> MIRLYPEQLRAQLNEGLRAAYLLLGNDPLLLQESQDAVRQVAAAQGFEEHHTFSIDPNTDWNAIFSLCQAMSLFASRQTLLLLLPENGPNAAINEQLLTLTGLLHDDLLLIVRGNKLSKAQENAAWFTALANRSVQVTCQTPEQAQLPRWVAARAKQLNLELDDAANQVLCYCYEGNLLALAQALERLSLLWPDGKLTLPRVEQAVNDAAHFTPFHWVDALLMGKSKRALHILQQLRLEGSEPVILLRTLQRELLLLVNLKRQSAHTPLRALFDKHRVWQNRRGMMGEALNRLSQTQLRQAVQLLTRTELTLKQDYGQSVWAELEGLSLLLCHKPLADVFIDG;>GPHMSYQVLARKWRPQTFADVVGQEHVLTALANGLSLGRIHHAYLFSGTRGVGKTSIARLLAKGLNCETGITATPCGVCDNCREIEQGRFVDLIEIDAASRTKVEDTRDLLDNVQYAPARGRFKVYLIDEVHMLSRHSFNALLKTLEEPPEHVKFLLATTDPQKLPVTILSRCLQFHLKALDVEQIRHQLEHILNEEHIAHEPRALQLLARAAEGSLRDALSLTDQAIASGDGQVSTQAVSAMLGTLDDDQALSLVEAMVEANGERVMALINEAAARGIEWEALLVEMLGLLHRIAMVQLSPAALGNDMAAIELRMRELARTIPPTDIQLYYQTLLIGRKELPYAPDRRMGVEMTLLRALAFHPRMPLPEPEVPRQ[3x];> GPHMRWYPWLRPDFEKLVASYQAGRGHHALLIQALPGMGDDALIYALSRYLLCQQPQGHKSCGHCRGCQLMQAGTHPDYYTLAPEKGKNTLGVDAVREVTEKLNEHARLGGAKVVWVTDAALLTDAAANALLKTLEEPPAETWFFLATREPERLLATLRSRCRLHYLAPPPEQYAVTWLSREVTMSQDALLAALRLSAGSPGAALALFQGDNWQARETLCQALAYSVPSGDWYSLLAALNHEQAPARLHWLATLLMDALKRHHGAAQVTNVDVPGLVAELANHLSPSRLQAILGDVCHIREQLMSVTGINRELLITDLLLRIEHYLQPGVVLPVPHL;>[2x]GPHMKFTVEREHLLKPLQQVSGPLGGRPTLPILGNLLLQVADGTLSLTGTDLEMEMVARVALVQPHEPGATTVPARKFFDICRGLPEGAEIAVQLEGERMLVRSGRSRFSLSTLPAADFPNLDDWQSEVEFTLPQATMKRLIEATQFSMAHQDVRYYLNGMLFETEGEELRTVATDGHRLAVCSMPIGQSLPSHSVIVPRKGVIELMRMLDGGDNPLRVQIGSNNIRAHVGDFIFTSKLVDGRFPDYRRVLPKNPDKHLEAGCDLLKQAFARAAILSNEKFRGVRLYVSENQLKITANNPEQEEAEEILDVTYSGAEMEIGFNVSYVLDVLNALKCENVRMMLTDSVSSVQIEDAASQSAAYVVMPMRL

Clamp loaders are pentameric ATPases that place circular sliding clamps onto DNA, where they function in DNA replication and genome integrity. Because the sliding clamp is a closed ring in solution, it needs to be opened and placed onto DNA by a separate ATPase complex called the clamp loader. All clamp loaders are pentameric ATPases of the AAA + family (ATPases associated with various cellular activities). Here we describe a series of structures of the E. coli clamp loader in the process of placing the clamp onto a p/t-junction.

The Closed-DNA1 and Closed-DNA2 structures reveal how the clamp closes and yields insight into sliding clamp release. By comparing the Open-DNAp/t and Closed-DNA1 structures we infer that the clamp closes through two motions. The sliding clamp subunit bound to A, B, and C moves laterally, while the second sliding clamp subunit bound to C, D, and E pivots down and in towards the A-gate. Despite this, the conformation of the clamp loader is essentially identical across Open-DNAp/t, Closed-DNA1, and Closed-DNA2. The only difference between Closed-DNA1 and Closed-DNA2 lies within the contacts between the clamp loader and the sliding clamp. In Closed-DNA1, all five subunits of the γ-complex contact the ß-clamp, although the D and E subunits lose substantial contact relative to the Open-DNAp/t state. We propose that the Closed-DNA1 conformation precedes the Closed-DNA2 conformation in a trajectory towards clamp release. In Closed-DNA1 and Closed-DNA2 structures, the clamp makes multiple direct contacts with DNA, primarily mediated by Gln15, Arg80, and Arg73 of clamp subunit I, and Gly23, Arg24, Arg80, and Gln149 of the second ß-clamp subunit. Previous work showed Arg24 and Gln149 of the ß-clamp are important for efficient loading. Our structures show that ATP hydrolysis is not strictly required for closure but is more likely to drive complete disengagement of the clamp loader.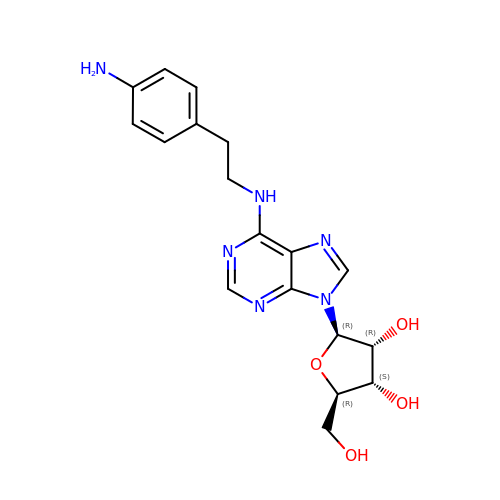N-[2-(4-aminophenyl)ethyl]adenosine | C18 H22 N6 O4 | XTPOZVLRZZIEBW-SCFUHWHPSA-N> MPVFHTRTIESILEPVAQQISHLVIMHEEGEVDGKAIPDLTAPVAAVQAAVSNLVRVGKETVQTTEDQILKRDMPPAFIKVENACTKLVQAAQMLQSDPYSVPARDYLIDGS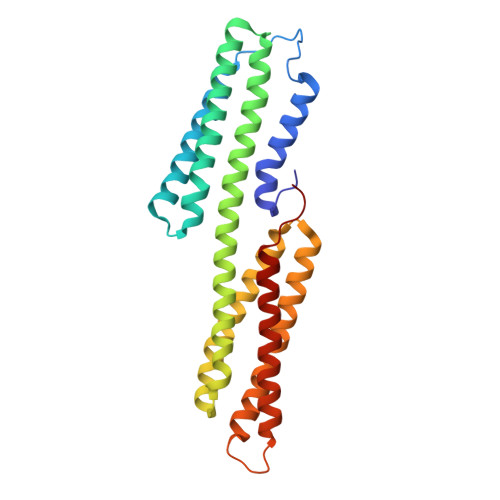RGILSGTSDLLLTFDEAEVRKIIRVCKGILEYLTVAEVVETMEDLVTYTKNLGPGMTKMAKMIDERQQELTHQEHRVMLVNSMNTVKELLPVLISAMKIFVTTKNSKNQGIEEALKNRNFTVEKMSAEINEIIRVLQLTSWDE> MSSWDRFDTPWDSIIDESTWEHYTFKYDASFEAFSSMEVDEDLTITVSVLFASTSDNTVTVGQVLGLTMDNRAGSYFGAGSSWTSEAAVNNEAGSGFQSSHALQLSYSVEDGVISSFGSEAFCSFYNTVSFESSSDVQAAVNSLYNLDVLFSSGSGDSEQHYVVFGETASFESLAEHETSSQYITHVECMFNSVVEFEVKTYDWGRPVKPVGSDWSTDTPVVGVWVNEIYNGNKDWGES;>[2x]MDKATLVKTIAYRMGNVKGQDTAIDFELALSIERLEGQEFVPWFLLSENNFFEGTAQENRIPVPRGFIREYEEGSLYLRRVAGTGK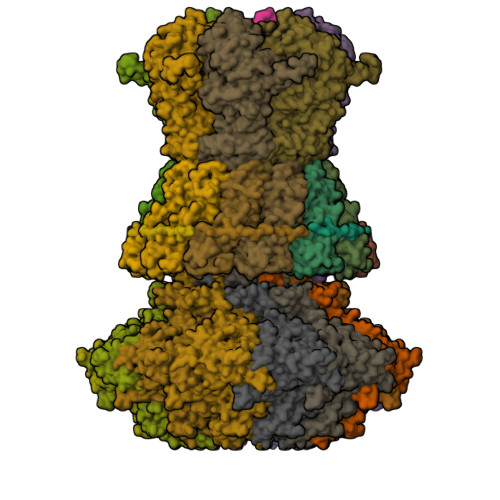CLIKKSQDQLLKYEGMTGEPSHYSLTNQYFRIYPVPQEDFKVELLFYRKSSTLNVEDNPWYEYAAELLVAETIWAMLSARRDKMADYWKSVAADQMRRLTILDAERRLANQEIFMG;> MEVTHKQFDLSGFLPDQAPDTLKSGAISRGFNVKPTILGWEKSGGFRETNTAPTNEKDFIFFWSPAIGDNRWFSGGDKTVQQVEGNVVSDVSRTGGYTAAAAARWNAVNFNGVLLMNNELDSPQYLAASGKLEDFPNLPSNVRFRTVAVYKNFILGLGVNFGSGFLDDEIYWSHQADPGTMPPNWDYANAASDSGRTPLPSEGYCVTSEELGSMNIVYKSDSIWTMQLIGGQWIFRFENKFPGQGILNKKSVVSFEGKHFVVTQKDIIVHDGYQVRSVADKRVRNFFFTDMNSDYFERVFVVKDPRVAEVYVFYPSKNSVDGLCDRALVWNWRDDVWSLLNLRPLKHAAYGYEITGVSITWDNFVGGWESTGLWQADEDVAKYAPVLHYSFRDVPKLLAPTPQALFIDEEIEAVWEREDIVIGSISRDGVPYQDYERNKSVSSISFDVDTTEPFDVYIGYKGSLEDSVEWEFAGTVNPMEDKRLFCLLTAGLFSMRIISKAQTFILRSYKITYEFAGEMWA;>[2x]MEILYTGASESLHSTILKALLERIDLGDTFISDNYTRWQATERYYMMYKIPNKKDKAAIEKWNKGDTDFKSLVMPYSYAQLMTAHAYMVNVFLNRDPIFQTDSLNGDGTERELALESMLQYQVKAGEMEPSLLVWFMDALRYGVGVLGDYWEEHVFHQTVFEVKKTRVVKGYEGCKTFNVMVYDFIPDPRVALCKYQEGEFFGRRLDLNVLDLKKGAKFGKYFNVEHAEALVAASKEEMYRRDPSIGQQRSLKDSTMTPKGKQVGDISCVEIFVRLVPKDWGLGDSEFPEMWVFTVADKKYIVAAEPVNTLDDKFPFHILECEIDGYMNKSRGLLEISAPMNDILTWLFDSHMYNKRQIMNNQFIGDPSALVVKDVESKEPGKFIRLRPIISQLPVTDVTAQNIQDVQVVERNMQRIVGVNDDVAGQSSPSSRRSATEFRGTTSFASSRLANLAYFFSVTGFRSLAKSLIVKTQQLYTVEMKVKVAGDNIKGAQSIIVKPEDISGQFDIMPVDGTLPVDRMAQAQFWMQIMSMVAGNPVLGAEYRLGDIFSYTARLAGLKGIDKMKIRILDDDQILALILA> GSSGSSGMFPAQEEADRTVFVGNLEARVREEILYELFLQAGPLTKVTICKDREGKPKSFGFVC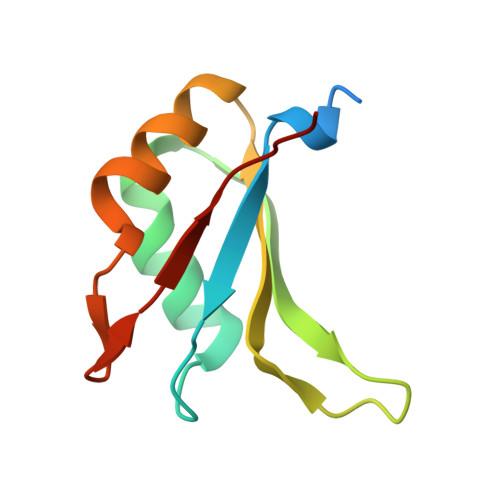FKHPESVSYAIALLNGIRLYGRPINVSGPSSG>[8x]HHHHHHVKLTLYGLDPSPPVRAVKLTLAALNLTYEYVN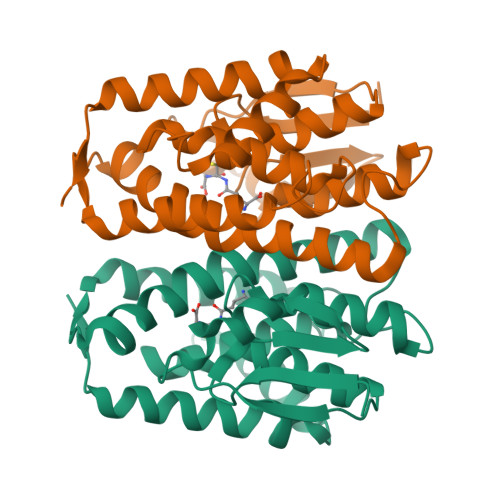VDIVARAQLSPEYLEKNPQHTVPTLEDDGHYIWDSHAIIAYLVSKYADSDALYPKDPLKRAVVDQRLHFESGVVFANGIRSISKSVLFQGQTKVPKERYDAIIEIYDFVETFLKGQDYIAGNQLTIADFSLVSSVASLEAFVALDTTKYPRIGAWIKKLEQLPYYEEANGKGVRQLVAIFKKTNFTFEA(4S,5R)-5-hydroxy-4-(3-hydroxyphenyl)-3,4,5,6,7,8-hexahydroquinazoline-2(1H)-thione 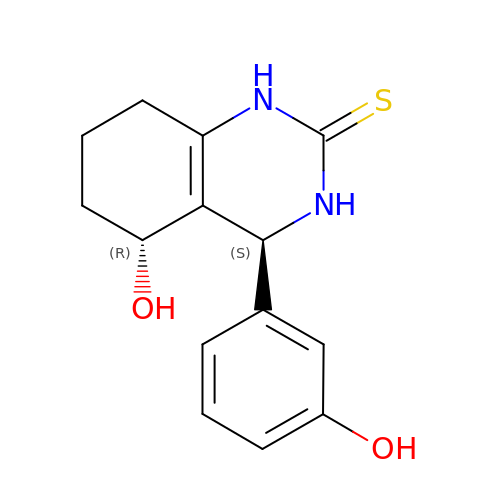| C14 H16 N2 O2 S | RZXURKNWIBRDDX-YPMHNXCESA-N> MNRIISINGPLVIAKGKFSIFEVVRVGEEKLIGEVIGIENDKAYIQVYEDTNGLKVGEPVFNTGKPLTIELGPGLLANIFDGLGRPLKDIYEKTQSIYIPKGIDLPTLDRKKVWEFIPKKKKGDTIKGGDIIGTVNENGFEHRIIVPPNVEGKIEEIYEGNFTIEETIAIVNGKPIKLYHEWPIRKPRPYKEKLDYNYPFITGTRVLDIMFPIAKGGSAAVPGPFGSGKTVLNQQIAKWADSDIVIYIGCGERGNEMTEVLEEFPKLKDPKTGKPLMYRTILIANTSNMPIAAREASIYLGATIGEYFRDQGYSVVVNADSTSRWAEALREISSRLGEIPSEEGYPAYLLRKLAEFYERSGRVRTLNDLEGSLTIIGAVSPPGGDFSEPVTQNTLRLVGALWALDSKLAYKRHYPAINYLISYTKQWEFVKKYFEELYEDVIEIREEFFAILKRESELMDIVSIVGPDALSDNEKIYLHMGRIIREGFLQQDAFDENDSYSPLEKTIELMRIIHKYYVTVKQLLGKIPLEEIEQKGIHEKIIKLRYKSLKEFREEIKAIEQEILSLLNSQ;> MPSIKPPLIAVELENPMLGEVIDLEETKAIVIAAYENKALALLFDYYTGEIKQINRQGNTYKIAVSEDYIGGIFNGFGEPIKGPKPYPEDYRDINGLAINPYARKVPNEILYTGISSIDVAHPLLKGQKIAIFSPPGLPMERLALQIARNVAKDKTIIFAAIGVPSDIYKMFIDEFINTKAIMNSAIFISKADSSPIEKIYTPRVALTLAEYLAFEKNRDVLVLMLDMTNYADALREISTLRKEIPSRRGYPAYLYTDLASIYERSGLTSKGSITLIPMLTMPGNDITHVVPDLTGYITEGQYV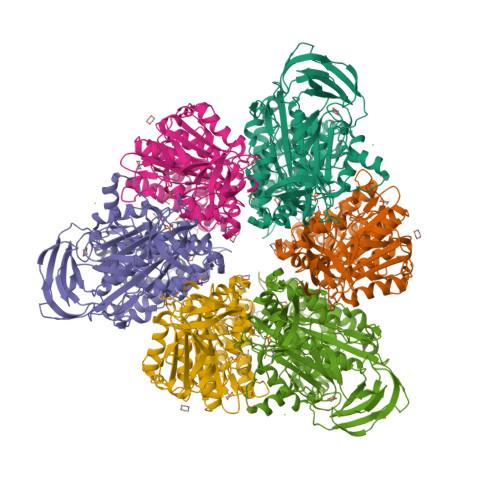LSQDLHSKNIYPPIDLLKSLSRLAKNGMSKKHKKYADILIKSYAKGLEARDIATIVGEDSLSKEDKAYLKFAELVEKEFIKQDYYEYRSIEKSFEIIDSILSQSGLPYSPIQ> AYERQYYPGATSVAANRRKHMSGKLEKLREISDEDLTAVLGHRAPGSDYPSTHPPLAEMGEPACSTRENVAATPGAAAGDRVRYIQFADSMYNAPATPYFRSYFAAINFRGVDPGTLSGRQIVEARERDMEQCAKVQMETEITDHALAGVRGATVHGHSVRLQEDGVMFDMLDRRRLENGTIIMDKDQVAIPLDRKVD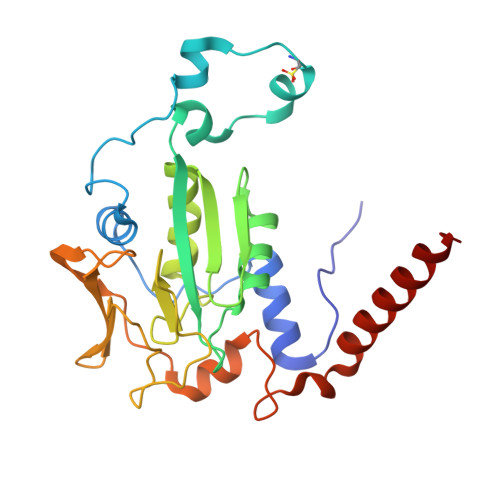LGKPMSSEEAAKRTTIYRVDNVAFRDDAEVVEWVHRIFDQRTKFGFQPK>[2x]TGCVLNKLFQLPTPPLSRHQLKRLEEHRYQSAGRSLLEPLMQGYWEWLVRRVPSWIAPNLITIIGLSINICTTILLVFYCPTATEQAPLWAYIACACGLFIYQSLDAIDGKQARRTNSSSPLGELFDHGCDSLSTVFVVLGTCIAVQLGTNPDWMFFCCFAGTFMFYCAHWQTYVSGTLRFGIIDVTEVQIFIIIMHLLAVIGGPPFWQSMIPVLNIQMKIFPALCTVAGTIFSCTNYFRVIFTGGVGKNGSTIAGTSVLSPFLHIGSVITLAAMIYKKSAVQLFEKHPCLYILTFGFVSAKITNKLVVAHMTKSEMHLHDTAFIGPALLFLDQYFNSFIDEYIVLWIALVFSFFDLIRYCVSVCNQIASHLHIHVFRIK

Choline/ethanolamine phosphotransferase 1 (CEPT1) catalyzes the last step of the biosynthesis of PC and PE in the Kennedy pathway by transferring the substituted phosphate group from CDP-choline/ethanolamine to diacylglycerol. CPT1, CEPT1 and EPT1 belong to the CDP-alcohol phosphotransferase (CDP-AP) family, whose members share a common property of catalyzing the transfer of a substituted phosphate group from a CDP-linked donor to an acceptor alcohol. CEPT1 is a dimer with 10 transmembrane segments (TMs) in each protomer. TMs 1-6 constitute a conserved catalytic domain with an interior hydrophobic chamber accommodating a PC-like density.

Eventually, the structure of hCEPT1 was determined to be 3.7 Å resolution using 459,021 particles. A lipid-like density was unambiguously observed in the structure of CEPT1, of which acyl tails reside in the hydrophobic chamber and the polar head is placed in the catalytic cavity. Because no lipid was added during protein purification or sample preparation, the density may indicate an endogenous lipid. However, a portion connecting the 3-OH group remains void, which is enough to accommodate a phosphocholine or phosphoethanolamine moiety. This observation suggests that the density belongs to a PC or PE molecule, the products of CEPT1. After fitting a PC molecule, the phosphate group is close to the carboxyl groups of four conserved aspartates on the CDP-binding motif, which coordinate two metal ions to stabilize the pyrophosphate of the CDP moiety in the bacterial homologs. CEPT1 prefers Mg2+ for PC production; therefore, we modeled two Mg2+ ions at similar positions to stabilize the phosphate group of PC in the structure. Two tails are coordinated in the hydrophobic chamber with hydrophobic residues, including Thr162/Val165/Val166/Thr169 of TM3, Cys185/Met192/Phe193 of TM4, Val213/Val216/Phe219/Ile220 of TM5, and Cys253/Thr254 of TM6. In addition, Gln217 seems to form a hydrogen bond with the carbonyl oxygen of the sn−1 acyl group. The trimethylammonium group may interact with the carboxyl group of Glu65 electrostatically. Two basic residues, His155 and His197, are close to the glycerol backbone of the endogenous PC molecule in our structure.>TRDQNGTWEMESNENFEGYMKALDIDFATRKIAVRLTQTKVIDQDGDNFKDKTTSTFRNYDVDFTVGVEFDEYTKSLDNRHVKALVT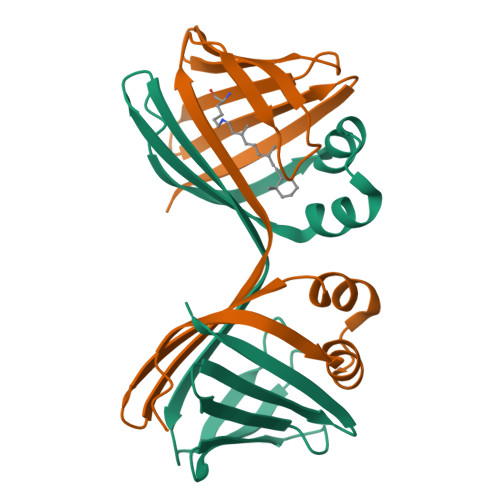WEGDVLVCVQKGEKENRGWKKWIEGDKLYLELTCGDQVCRQVFKKK[12x]HOMOSERINE 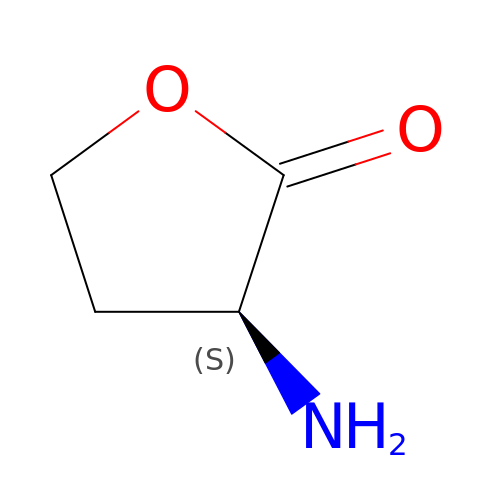LACTONE | C4 H7 N O2 | QJPWUUJVYOJNMH-VKHMYHEASA-N>[3x]ETGIDWDVFCSQNENIPAKFISRLVAPKCLAV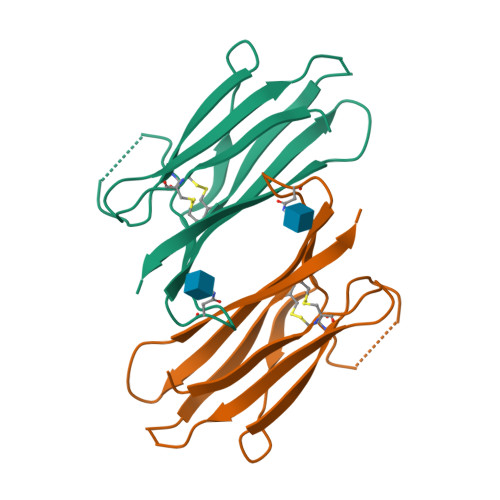EKMDVDCSNGLVPITHEHGFNMMLIQYTRNKLLDSPGMCVFWGPYSVPKNDTVVLYTVTARLKWSEGPPTDLSIQCYMPKSPDAPKPEACLAAPLEHHHHHH>[2x]GAQPADFQAEVESDTRIQLSWLLPPQERIIMYELVYWAAEDEDQQHKVTFDPTSSYTLEDLKPDTLYRFQLAARSDMGVGVFTPTIEARTAQSTPSAPPQK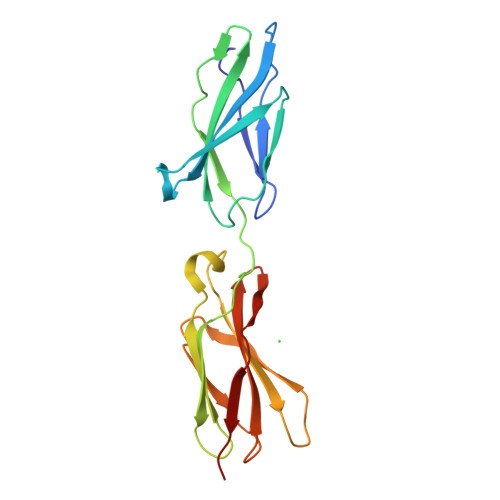VMCVSMGSTTVRVSWVPPPADSRNGVITQYSVAYEAVDGEDRGRHVVDGISREHSSWDLVGLEKWTEYRVWVRAHTDVGPGPESSPVLVRTDED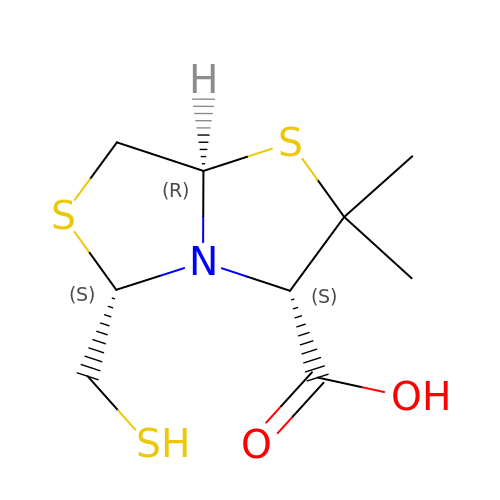(3S,5S,7aR)-2,2-dimethyl-5-(sulfanylmethyl)tetrahydro[1,3]thiazolo[4,3-b][1,3]thiazole-3-carboxylic acid | C9 H15 N O2 S3 | IKSIYRPSHTUWIX-XVMARJQXSA-N5-(4-fluorophenyl)thieno[2,3-d]pyrimidin-4(3H)-one | C12 H7 F N2 O S | 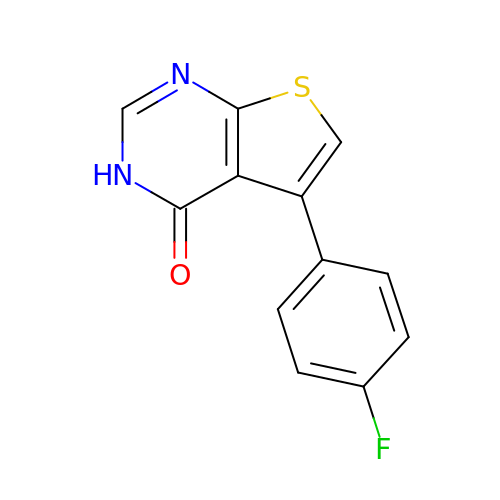DARIIFLATJJEOB-UHFFFAOYSA-N>[4x]HHHHHHMEPACKYDFATSVLFTEAELHTRMRGVAQRIADDYSNCNLKPLENPLVIVSVLKGSFVFTADMVRILGDFGVPTRVEFLRASSYGHDTKSCGRVDVKADGLCDIRGKHVLVLEDILDTALTLREVVDSLKKSEPASIKTLVAIDKPGGRKIPFTAEYVVADVPNVFVVGYGLDYDQSYREVRDVVILKPSVYETWGKELERRKAAGEAKR

One potential new drug target is 6-oxopurine phosphoribosyltransferase (PRTase), an enzyme central to the purine salvage pathway and whose activity is critical for the production of the nucleotides (GMP and IMP) required for DNA/RNA synthesis within this protozoan parasite. For example, T. brucei has three 6-oxopurine PRTase isoforms whereas there is only one 6-oxopurine PRTase in humans. These enzymes catalyze the transfer of the ribose 5'-phosphate moiety from 5-phospho-α-D-ribosyl-1-pyrophosphate (PRib-PP) to their respective purine bases (hypoxanthine, guanine or xanthine). Here, we show that two of the three T. brucei isoforms of the 6-oxopurine PRTases are identified as HGPRTs as a reflection of their substrate preference for hypoxanthine and guanine and the third isoform is identified as HGXPRT reflecting that it uses all three naturally occurring bases. In both enzymes, the active site is situated at the interface of two domains referred to as the hood and core and is primarily comprised of three pockets identified as the purine base binding pocket, the 5′-phosphate binding pocket and the pyrophosphate (PPi) binding pocket.

To explain the mode of binding of the ANPs, crystal structures of HGPRT-I in complex with compounds 1, 2, 6 and 7, and HGXPRT in complex with compounds 2 and 7 were determined. For compounds 2 and 7, we have determined structures of complexes with both HGPRT-I and HGXPRT, thus allowing a direct comparison of the binding modes of these two ANPs. However, compound 2 binds differently to the two enzymes. In the HGPRT-I.2 complex the phosphonate attach to the linker occupies the 5´-phosphate pocket and the phosphonate connected to the attachment occupies the PPi pocket. However, in the HGXPRT.2 complex the situation is reversed and the phosphonate attached to the linker occupies the PPi pocket and the phosphonate of the attachment occupies the 5´-phosphate pocket. Although the phosphonate groups are swapped in the two structures the hydrogen bonding networks in the 5´-phosphate pocket are virtually identical in the two complexes. In the PPi pocket, the phosphonate groups are oriented at slightly different angles in the two structures, this is due to the fact that the linkers/attachments are different and the presence of Mg2+ in the HGPRT-I complex. Nonetheless, both binding modes result in the L53-K54/L86-K87 peptide bond adopting a cis conformation. In this location, there are fewer interactions between the compound 2 and HGXPRT compared to HGPRT-I and this difference is the likely reason for this compound having a higher Ki value for HGXPRT compared to HGPRT-I (6.54 μM vs 0.11 μM). By contrast, the binding of compounds 1 and 2 is very similar in HGPRT-I and human HGPRT.> DVVVQAPTQVPGFLGDSVTLPCYLQVPNMEVTHVSQLTWARHGESGSMAVFHQTQG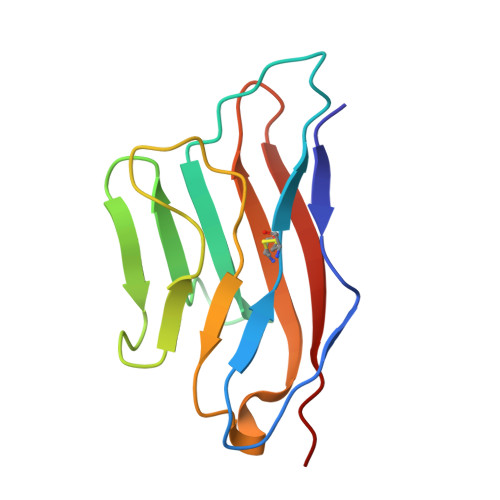PSYSESKRLEFVAARLGAELRNASLRMFGLRVEDEGNYTCLFVTFPQGSRSVDIWLRVLA>TRDQNGTWEMESNENFEGYMKALDIDFATRKIAVRLTQTLVIDQDGDNFKTKTTSTFRNYDVDFTVGVEFDEYTKSLDN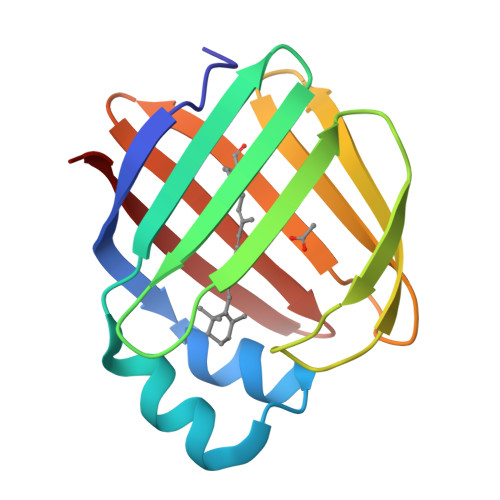RHVKALVTWEGDVLVCVQKGEKENRGWKKWIEGDKLYLELTCGDQVCRQVFKKK[2x]> MGHHHHHHSMI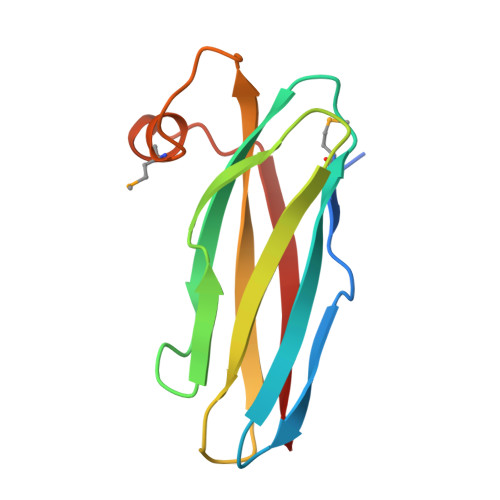NVDPPTGNYPATGGNSTHNITSESDSRLAFKVKSSNNEHYRVRPVYGFVDAKGKSKLDINRLPGPPKEDKIVIQYAEVPAEETDPMAPFKAGAQQGEIIVKLIAA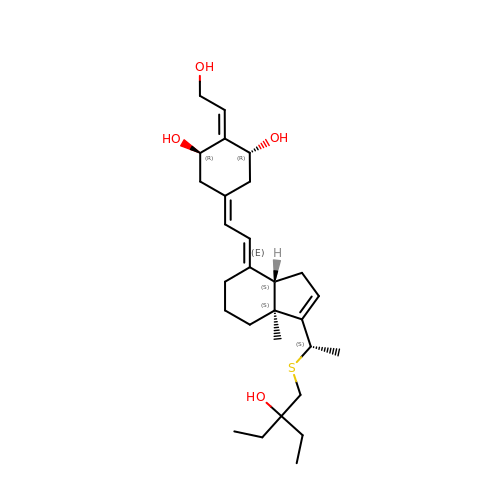(1R,2E,3R,5Z,7E)-17-{(1S)-1-[(2-ethyl-2-hydroxybutyl)sulfanyl]ethyl}-2-(2-hydroxyethylidene)-9,10-secoestra-5,7,16-triene-1,3-diol | C28 H44 O4 S | PIRFBNFXEQEXIT-NSHLMRFWSA-N> MSAPTPLAEASQIPTIPALSPLTAKQSKGNFFSSNPISSFVVDTYKQLHSHRQSLELVNPGTVENLNKEVSRDVFLSQYFFTGLRADLNKAFSMNPAFQTSHTFSIGSQALPKYAFSALFANDNLFAQGNIDNDLSVSGRLNYGWDKKNISKVNLQISDGQPTMCQLEQDYQASDFSVNVKTLNPSFSEKGEFTGVAVASFLQSVTPQLALGLETLYSRTDGSAPGDAGVSYLTRYVS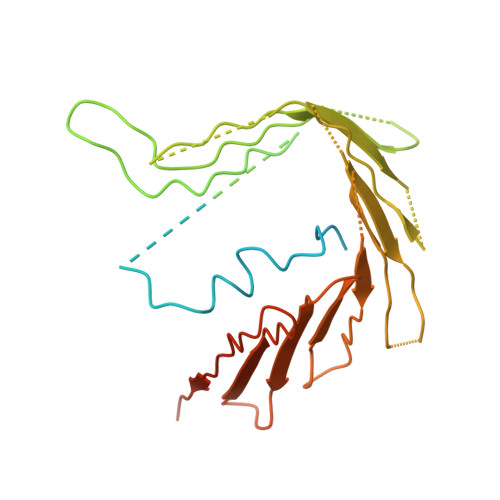KKQDWIFSGQLQANGALIASLWRKVAQNVEAGIETTLQAGMVPITDPLMGTPIGIQPTVEGSTTIGAKYEYRQSVYRGTLDSNGKVACFLERKVLPTLSVLFCGEIDHFKNDTKIGCGLQFETAGNQELLMLQQGLDADGNPLQALPQL> WSHPQFEKTAGRRKVQVSYVIRDEVEKYNRNGVNALQLDPALNRLFTAGRDSIIRIWSVNQHKQDPYIASMEHHTDWVNDIVLCCNGKTLISASSDTTVKVWNAHKGFCMSTLRTHKDYVKALAYAKDKELVASAGLDRQIFLWDVNTLTALTASNNTVTTSSLSGNKDSIYSLAMNQLGT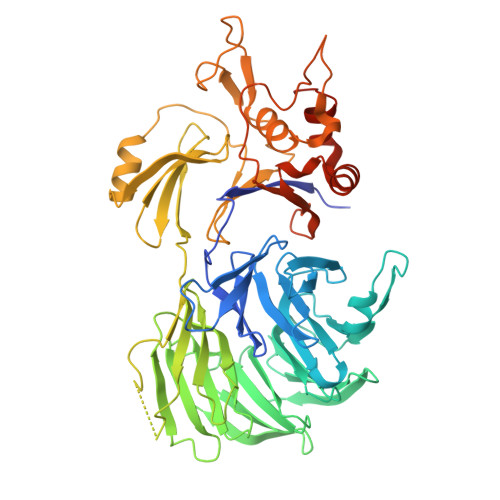IIVSGSTEKVLRVWDPRTCAKLMKLKGHTDNVKALLLNRDGTQCLSGSSDGTIRLWSLGQQRCIATYRVHDEGVWALQVNDAFTHVYSGGRDRKIYCTDLRNPDIRVLICEEKAPVLKMELDRSADPPPAIWVATTKSTVNKWTLKGIHNFRASGDYDNDCTNPITPLCTQPDQVIKGGASIIQCHIFNDKRHILTKDTNNNVAYWDVLKACKVEDLGKVDFEDEIKKRFKMVYVPNWFSVDLKTGMLTITLDESDCFAAWVSAKDAGFSSPDGSDPKLNLGGLLLQALLEYWPRTHVNPMDEEENEVNHVNGEQENRVQKGNGYFQVPPHTPVIFGEAGGRTLFRLLCRDSGGETESMLLNETVPQWVIDITVDKNMPKFNKIPFYLQPHASSGAKTL> MSSVIREIAKRFLEQATINIAEEVVREYGDHERTMISVGVHFQACCLISDEYTLEDETTPRYVLLEGLKRQEAISKQNNICSTLGLEPLRNLADIFDRKTRRFLEVGITKRESDEYYQEKFNKIGNDMDIHVFTYEGKYFSNNPNGLEDIQKTRIFTFLSFVSDELRKENMFTEMYVTEEGAPELEMYKSKLFIAMRDESVPLPYINYEHLRTRCETFKRNQAECEAKVADVASRLKIKLEHLEENKLRPLEIPKEKEAPYTHKFLMKDAWFFAKPHDSERAQPQQILYDFFEAANMGFMTTSPKPIFGKQGLMYHSLWGQTKRAIKDKRNELEPSEQRDFLCGIGRASKKIQEDKWQESREEEFKQEETKGAAKRGFPTWFNEEWLWAMRDSGDGDNKIGDWIPMAEMPPCKNEMEDYAKKMCEELESKIQGTNCAREMSKLIHTIGSLHTECRNFPGKVKIVPIYCRGTLRGESTDCLFGIAIKGKSHLNKDDGMYTVVTFEFSTEEPNPSKHEKYTVFEAGTVPVEAVVLTPKRERVLKEKKLFLYCRTTGMSKLKNDWFSKCRRCLIPTMETVEQIVLKECALKEENRVSEMLENKRAWIAHENGENLTRLVSTKLKDLCRMLIVTQFYYCIYNDNQLEGFCNEQKKFLMFLQADKDSKSAFTFNQKGLYEKIEECIVSNPLCIFLADRLNKLFLVAKSNGAKYFE;> MEINPYLLMLNNDITSMISLTYPYTGAPPMSHGTSTKYSMETVSRTYSYSRTKKEVPSGIFPIERRKFCNTIEDKENLEKPNGNVDINFMLSLAEMLEEKMGKGFFKFCANEAEAEILKMHFSKLTEGRQTYDWTSERNMPAATALQLTVDAIQETQGTFKGTTMVEYCNKILEMMDWPEVKFKKVRMIVQRHWDPKTKKEIKMKSPTLMITKIGREEFIKRICTINTMAKDGERGKYKRRAIATPGMGIRPFSKIVETLAQKICERLAESGLPVGGNEKKAKLKTTVSSTNSKLQEGQFMVNITGDNSKWNECQQPEAYLAMLAYITKDSSNLMKDLCSVAPTLFCNKYVKMGQGFRAKNKRKTKEIVIPAKKMKERKELMNAEWRDLFETIEPYMDGECCFLGGGMLMGMFNMLSTVFGVMTLNYREEALARRNCYWTGLQSSDDFVLFCISRTWPEMEMTILKFIAVCKLMGINMSLEKSYGCLPELFEFTSMFFSGDFVSNIALELPAFTTAGMNEGTDFTAAMSV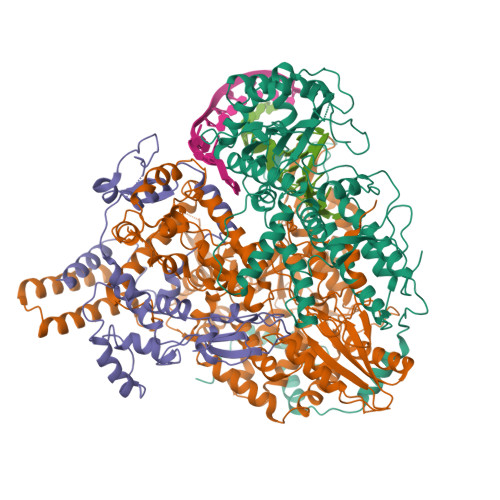IRTNMINNGLSPGTALMALRICLQEFRATYRVHPYDSGVKNHRMKIIRKFIETIENKDGLLISDGGKLMNNISSLHIPEEILKEDLMDPSYRNRVFNPRNPFTQFEKTVDIFKASGPIRVEENEAVVSTHSFRTRSNRTLLNTDMRAMALEEKRYQVVCNMYRSVFESADVNTPIGSMSMGEAIEAKILDRARTQFENGIIGGEEYSEIKRLIEDAKRQRLSV;> MSLLLTLAKEYANLTKDKKSCKLLSQGTVSSYTTFKKWTTSRKEKNPSLRMRWAMGSKFPIMANREILEEAGIPEQWEGIDLWSKKDDVSKLGMVLASPAAITYWNFCGPGVDNSSVIKDVYKAKFMKKERWRETLWGPMNFELVGKQRRVVETQPVEIKLNQKEIKELTMWVLFEDEANLASKFIQENFSLVLSLRELYKGKAVNKDVAAFMIAHQFSPEKRFLPTFGPIRPERMELLHCLGGDFWKIEAVTAGSLNEEQKKRDVRAVARKICLRASVDLFTPAEKIRDYIASVTMRFGTVERTFEDVIRNSDDISAEVTLCKAALGCELGKSMSFGNLNLRKVSGEAETMEKTVYWGLKPIKYKCWRGEETFYCELRKVTCMFRRSEGLDWANIGPGSPEERRELLAMVMIFCRDGRFFESAPVNIDESFFRTRLNKEIPYQYVLLKWVRQSRDNLDALLSTRGLIPAHIGQFGKGMGIDGSSSSSMVYKGVMLSKTPIDIVESKEKHRLFLNDNIEAVTERGAMVASIMDLSEDNRETFNDVTFNHVDLAVLKDEKTAIIKIYRSLVERINTDDDGLPALIMGKRYLELYQLDEVKDAVGLIPKRMLGAYSYQARQLIQSQIKNDSYSLPEIIKLLPFCYSPPKKMLFDGTFHFKNQMYVRPGINTNLFSFSKTDKSKIYVNGSAVKIKLVLGDDEMDTSLAFVEGFQVCEYDPRAPLIPRRDLRLIGFGKKVRVFVGQGQEKTLVRTSSKRAASHDVSKNIRRMRLEV We reconstituted the biosynthesis of the benzoxazole moiety found in nataxazole by adding two enzymes (NatL2, NatAM), to 3‐HAA, ATP, and Mg2+. We have determined the structures of both NatL2 (homologue of BomJ) and NatAM (homologue of BomN) from the antitumor nataxazole pathway. We show NatL2 catalyzes ester not, as previously reported, amide formation; the amide is a shunt product. NatAM catalyzes benzoxazole from this ester by a mechanism that we propose involves shuttling of protons to control the fate of a hemiorthoamide intermediate.

We determined the 1.9 Å‐resolution crystal structure of NatL2 in the presence of ATP. NatL2 consists of two subunits in one asymmetric unit that PISA46 indicates form a homodimer. The individual monomers of NatL2 are structurally equivalent and can be superimposed with a root mean square deviation (rmsd) of 0.348 Å over 420 Cα atoms. Residues 5–436 in chain A and 1–322, 327–436 in chain B were traced. Residual electron density in both monomers was best modelled as AMP not ATP. NatL2 has an N‐terminal domain (1–320), a C‐terminal domain (326–404), and a C‐terminal extension (405–436). The N‐terminal domain, which binds AMP, forms an αβαβα structure with an additional β‐hairpin. A tetrahedrally coordinated zinc (Cys248, Cys308, Cys310, His254) is found in the N‐terminal domain over 20 Å away from AMP. In NatL2, the adenine ring is sandwiched between the main chain peptide bonds of Ala212 to Pro214 on one side and Tyr236 on the other. The C‐terminal extension (405–436) is a novel feature of NatL2 and has an extended strand followed by a turn and a shorter strand that reaches across to the other monomer filling a pocket in other monomer's C‐terminal domain below the AMP binding site.

> MSRSRPELGDWSSPAELAELQRSQLPRVLAQALRSPFYAARYRGTTPPRTADDFAGVEVTAKQDLRDQYPFGMLAVGREHLATYHESSGTAGEPTASYYTEEDWTDLAERFARKWTGIHPSDTFLVRTPYGLVITGHLAQAAGRLRGATVVPGDARSLATPLSRMVRVLKTLDVTLTWCNPTEITMLAAAAKAAGLRPDQDFPHLRAMFTAAEPLTEVRRRRLSEIWGGIPVVEEYGSTETGTIAGQCPEGRMHLWADRAIFEVYDPRTGTLSEAGRGQMVVTPLYRDAMPLLRYNLADDVEVSTDPCGCGWLLPTVTVLGRAGTGHRIGPATVTQQRLEELVFSLPAAYEVMFWRAKAHPDVLELEFEAPEPVRQRAVKELGAALDRELGVPHRITGLAPGTLVPAEALTAQRDILKARYLFAEDEDWDKAVMYF;> AMSRSRPELGDWSSPAELAELQRSQLPRVLAQALRSPFYAARYRGTTPPRTADDFAGVEVTAKQDLRDQYPFGMLAVGREHLATYHESSGTAGEPTASYYTEEDWTDLAERFARKWTGIHPSDTFLVRTPYGLVITGHLAQAAGRLRGATVVPGDARSLATPLSRMVRVLKTLDVTLTWCNPTEITMLAAAAKAAGLRPDQDFPHLRAMFTAAEPLTEVRRRRLSEIWGGIPVVEEYGSTETGTIAGQCPEGRMHLWADRAIFEVYDPRTGTLSEAGRGQMVVTPLYRDAMPLLRYNLADDVEVSTDPCGCGWLLPTVTVLGRAGTGHRIGPATVTQQRLEELVFSLPAAYEVMFWRAKAHPDVLELEFEAPEPVRQRAVKELGAALDRELGVPHRITGLAPGTLVPAEALTAQRDILKARYLFAEDEDWDKAVMYF> QQIEQPYRTGYHFQPPSNWMNDPNGPMLYQGVYHFFYQYNPYAATFGDVIIWGHAVSYDLVNWIHLDPAIYPTQEADSKSCWSGSATILPGNIPAMLYTGSDSKSRQVQDLAWPKNLSDPFLREWVKHPKNPLITPPEGVKDDCFRDPSTAWLGPDGVWRIVVGGDRDNNGMAFLYQSTDFVNWKRYDQPLSSADATGTWQCPDFYPVPLNSTNGLDTSVYGGSVRHVMKAGFEGHDWYTIGTYSPDRENFLPQNGLSLTGSTLDLRYDYGQFYASKSFFDDAKNRRVLWAWVPETDSQADDIEKGWAGLQSFPRALWIDRNGKQLIQWPVEEIEELRQNQVNLQNKNLKPGSVLEIHGIAASQADVTISFKLEGLKEAEVLDTTLV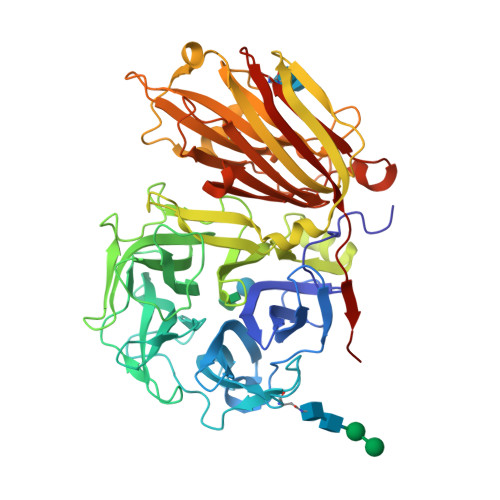DPQALCNERGASSRGALGPFGLLAMASKDLKEQSAIFFRVFQNQLGRYSVLMCSDLSRSTVRSNIDTTSYGAFVDIDPRSEEISLRNLIDHSIIESFGAGGKTCITSRIYPKFVNNEEAHLFVFNNGTQNVKISEMSAWSMKNAKFVVDQSVKSAA>[2x]MGHHHHHHMTKIKWLGAFALVFVMLLGGCSLPGLG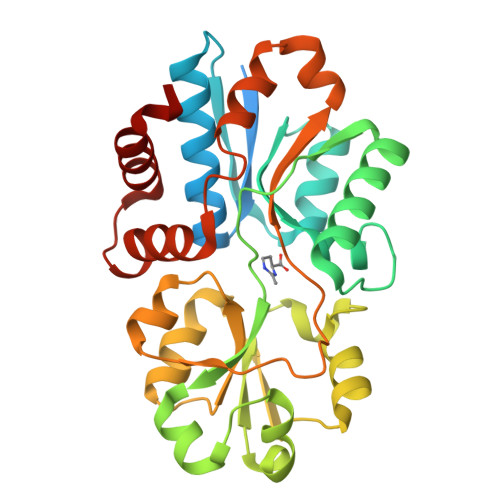GASDDTIKIGAQSMTESEIVANMIAQLIEHDTDLNTALVKNLGSNYVQHQAMLGGDIDISATRYSGTDLTSTLGKEAEKDPKKALNIVQNEFQKRFSYKWFDSYGFDNTYAFTVTKKFAEKEHINTVSDLKKNASQYKLGVDNAWLKRKGDGYKGFVSTYGFEFGTTYPMQIGLVYDAVKNGKMDAVLAYSTDGRIKAYDLKILKDDKRFFPPYDCSPVIPEKVLKEHPELEGVINKLIGQIDTETMQELNYEVDGKLKEPSVVAKEFLEKHHYFD>MSEAIVVNNQNDQSRAYAIPLEDIDVSNPELFRDNTMWGYFERLRREDPVHYCKDSLFGPYWSVTKFKDIMQVETHPEIFSSEGNITIMESNAAVTLPMFIAMDPPKHDVQRMAVSPIVAPENLAKLEGLIRERTGRALDGLPINETFDWVKLVSINLTTQMLATLFDFPWEDRAKLTRWSDVATALVGTGIIDSEEQRMEELKGCVQYMTRLWNERVNVPPGNDLISMMAHTESMRNMTPEEFLGNLILLIVGGNDTTRNSMTGGVLALN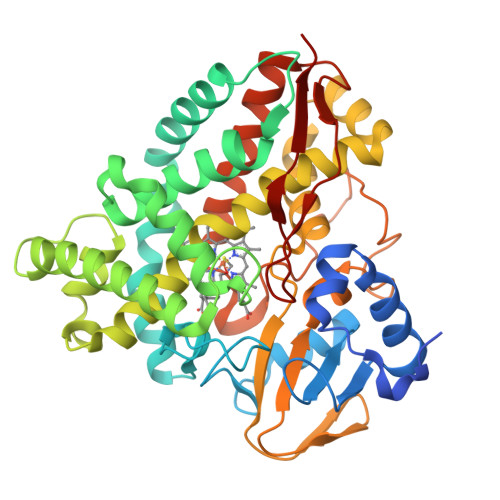ENPDEYRKLCANPALIASMVPEIVRWQTPLAHMRRTALQDTELGGKSIRKGDKVIMWYVSGNRDPEAIENPDAFIIDRAKPRHHLSFGFGIHRCVGNRLAELQLRIVWEELLKRWPNPGQIEVVGAPERVLSPFVKGYESLPVRINA[6x]>[2x]AKVFQWFGSNESGAEFGSQNLPGVEGKDYIWPDPNTIDTLISKGMNIFRVPFMMERLVPNSMTGSPDPNYLADLIATVNAITQKGAYAVVDPHNYGRYYNSIISSPSDFQTFWKTVASQFASNPLVIFDTNNAYHDMDQTLVLNLNQAAIDGIRSAGATSQYIFVEGNSWTGAWTWTNVNDNMKSLTDPSDKIIYEMHQY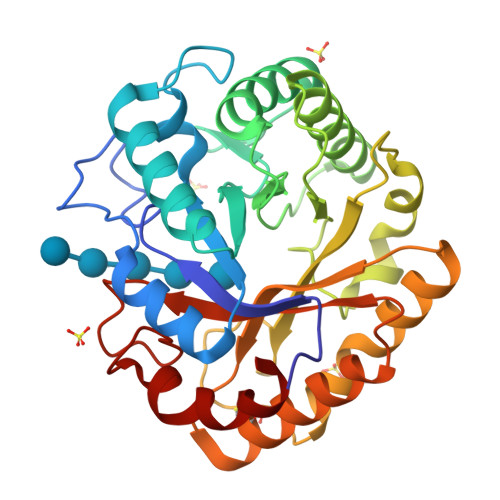LDSDGSGTSATCVSSTIGQERITSATQWLRANGKKGIIGEFAGGANDVCETAITGMLDYMAQNTDVWTGAIWWAAGPWWGDYIFSMEPDNGIAYQQILPILTPYL> MLEEALAAIQNARDLEELKALKARYLGKKGLLTQEMKGLSALPLEERRKRGQELNAIKAALEAALEAREKALEEAALKEALERERVDVSLPGASLFSGGLHPITLMERELVEIFRALGYQAVEGPEVESEFFNFDALNIPEHHPARDMWDTFWLTGEGFRLEGPLGEEVEGRLLLRTHTSPMQVRYMVAHTPPFRIVVPGRVFRFEQTDATHEAVFHQLEGLVVGEGIAMAHLKGAIYELAQALFGPDSKVRFQPVYFPFVEPGAQFAVWWPEGGKWLELGGAGMVHPKVFQAVDAYRERLGLPPAYRGVTGFAFGLGVERLAMLRYGIPDIRYFFGGRLKFLEQFKGVL;> MRVPFSWLKAYVPELESPEVLEERLAGLGFETDRIERVFPIPRGVVFARVLEAHPIPGTRLKRLVLDAGRTVEVVSGAENARKGIGVALALPGTELPGLGQKVGERVIQGVRSFGMALSPRELGVGEYGGGLLEFPEDALPPGTPLSEAWPEEVVLDLEVTPNRPDALGLLGLARDLHALGYALVEPEAALKAEALPLPFALKVEDPEGAPHFTLGYAFGLRVAPSPLWMQRALFAAGMRPINNVVDVTNYVMLERAQPMHAFDLRFVGEGIAVRRAREGERLKTLDGVERTLHPEDLVIAGWRGEESFPLGLAGVMGGAESEVREDTEAIALEVACFDPVSIRKTARRHGLRTEASHRFERGVDPLGQVPAQRRALSLLQALAGARVAEALLEAGSPKPPEAIPFRPEYANRLLGTSYPEAEQIAILKRLGCRVEGEGPTYRVTPPSHRLDLRLEEDLVEEVARIEGYETIPLALPAFFPAPDNRAVEAPYRKEQRLREVLSGLGFQEVYTYSFMDPEDARRFRLDPPRLLLLNPLAPEKAALRTHLFPGLVRVLKENLDLDRPERALLFEVGR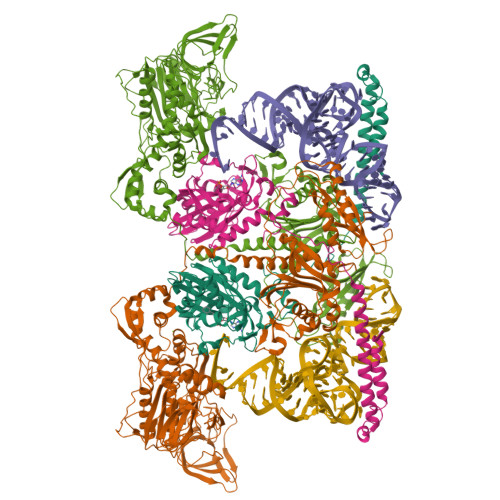VFREREETHLAGLLFGEGVGLPWAKERLSGYFLLKGYLEALFARLGLAFRVEAEAFPFLHPGVSGRVLVEGEEVGFLGALHPEIAQELELPPVHLFELRLPLPDKPLAFQDPSRHPAAFRDLAVVVPAPTPYGEVEALVREAAGPYLESLALFDLYQGPPLPEGHKSLAFHLRFRHPKRTLRDEEVEEAVSRVAEALRARGFGLRGLDTP> MITSALHRAADWAKSVFSSAALGDPRRTARLVNVAAQLAKYSGKSITISSEGSKAAQEGAYRFIRNPNVSAEAIRKAGAMQTVKLAQEFPELLAIEDTTSLSYRHQVAEELGKLGSIQDKSRGWWVHSVLLLEATTFRTVGLLHQEWWMRPDDPADADEKESGKWLAAAATSRLRMGSMMSNVIAVCDREADIHAYLQDKLAHNERFVVRSKHPRKDVESGLYLYDHLKNQPELGGYQISIPQKGVVDKRG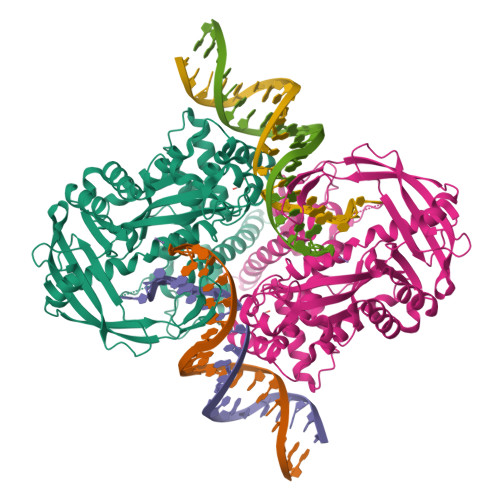KRKNRPARKASLSLRSGRITLKQGNITLNAVLAEEINPPKGETPLKWLLLTSEPVESLAQALRVIDIYTHRWRIEEFHKAWKTGAGAERQRMEKPDNLERMVSILSFVAVRLLQLRESFTPPQALRAQGLLKEAEHVESQSAETVLTPDECQLLGYLDKGKRKRKEKAGSLQWAYMAIARLGGFMDSKRTGIASWGALWEGWEALQSKLDGFLAAKDLMAQGIKIG> GPGSEFEPEKEEIRERYELSEKMLSACNLLKYNIKDPKALASKDMRICLNTLQHDWFRVSSQKSAVPAMVGDYIAAFEAVSPDVLRYIINMADGNGNTALHYSVSHSNFQIVKLLLDADVCNVDHQNKAGYTPIMLAALAAVEAEKDMQVVEELFSCGDVNAKASQAGQTALMLAVSHGR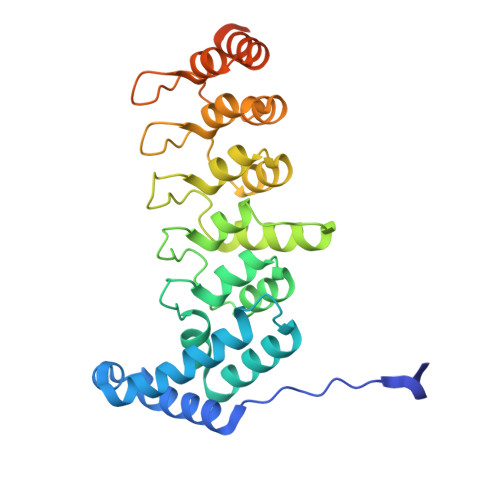IDMVKGLLACGADVNIQDDEGSTALMCASEHGHVEIVKLLLAQPGCNGHLEDNDGSTALSIALEAGHKDIAVLLYAHLNFSKAQSPSTPRLGRKTSPGPTHRGSFD> QPIFLNVLEAIEPGVVCAGHDNNQPDSFAALLSSLNELGERQLVHVVK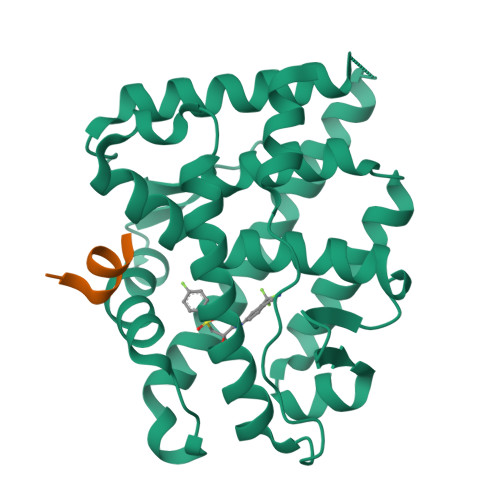WAKALPGFRNLHVDDQMAVIQYSLMGLMVFAMGWRSFTNVNSAMLYFAPDLVFNEYRMHKSRMYSQCVRMRHLSQEFGWLQITPQEFLCMKALLLFSIIPVDGLKNQKFFDELRMNYIKELDRIIACKRKNPTSCSRRFYQLTKLLDSVQPIARELHQFTFDLLIKSHMVSVDFPEMMAEIISVQVPKILSGKVKPIYFHTQ;> NTTDTLFSQHYR>MMAGPLSGLRVVELAGIGPGPHAAMILGDLGADVVRIDRPSSVDGISRDAMLRNRRIVTADLKSDQGLELALKLIAKADVLIEGYRPGVTERLGLGPEECAKVNDRLIYARMTGWGQTGPRSQQAGHDINYISLNGILHAIGRGDERPVPPLNLVGDFGGGSMFLLVGILAALWERQSSGKGQVVDAAMVDGSSVLIQMMWAMRATGMWTDTRGANMLDGGAPYYDTYECADGRYVAVGAIEPQFYAAMLAGLGLDAAELPPQNDRARWPELRALLTEAFASHDRDHWGAVFANSDACVTPVLAFGEVHNEPHIIERNTFYEANGGWQPMPAPRFSRTAS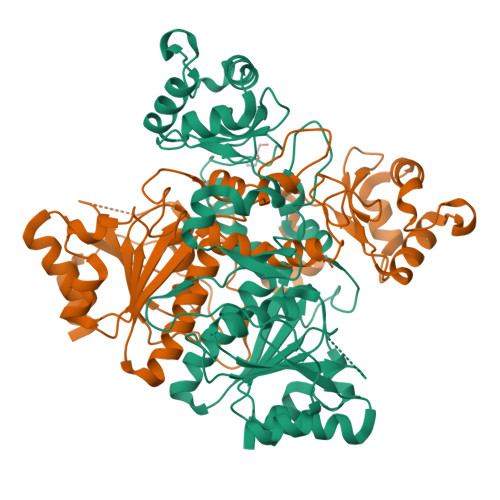SQPRPPAATIDIEAVLTDWDGGSGC[2x]> MVLSDKELFAINKKAVEQGFNVKPRLNYNTVSGVNGPLVILEKVKFPRYNEIVNLTLPDGTVRQGQVLEIRGDRAIVQVFEGTSGIDVKKTTVEFTGESLRIPVSEDMLGRIFDGSGRPIDNGPKVFAEDYLDINGSPINPYARIYPEEMISTGVSAIDTMNSIARG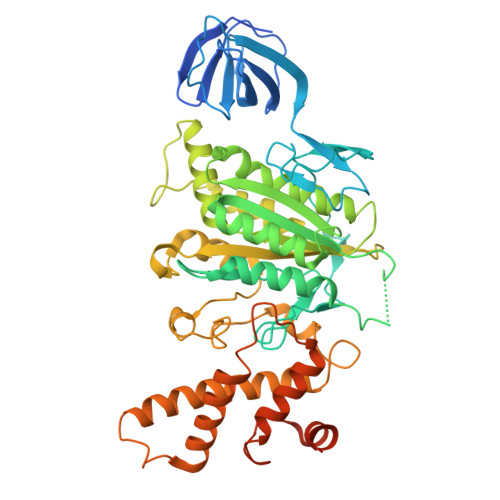QKIPIFSASGLPHNEIAAQICRQAGLVRPTKDVHDGHEENFSIVFAAMGVNLETARFFKQDFEENGSLERTSLFLNLANDPTIERIITPRLALTTAEYLAYQTERHVLTILTDMSSYADALREVSAAREEVPGRRGYPGYMYTDLSTIYERAGRVEGRNGSITQIPILTMPNDDITHPIPDLTGYITEGQIFVDRQLHNKGIYPPINVLPSLSRLMKSAIGEGMTRKDHGDVSNQLYAKYAIGKDAAAMKAVVGEEALSIEDKLSLEFLEKFEKTFITQGAYEDRTVFESLDQAWSLLRIYPKEMLNRISPKILDEFYDRARDDADEDEEDPDTRSSGKKKDASQEESLI> MNKESKDDDMSLGKFSFSHFLYYLVLIVVIVYGLYKLFTGHGSDINFGKFLLRTSPYMWANLGIALCVGLSVVGAAWGIFITGSSMIGAGV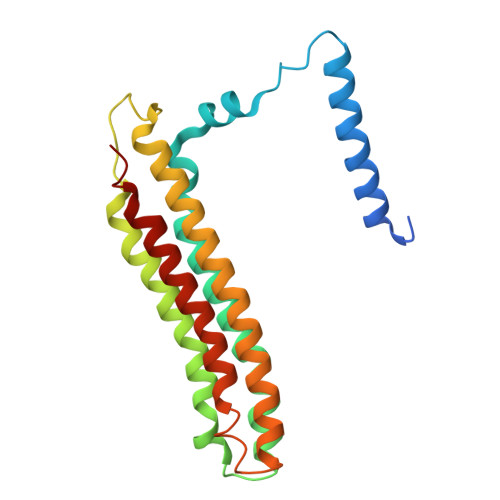RAPRITTKNLISIIFCEVVAIYGLIIAIVFSSKLTVATAENMYSKSNLYTGYSLFWAGITVGASNLICGIAVGITGATAAISDAADSALFVKILVIEIFGSILGLLGLIVGLLMAGKASEFQ Protein-engineering methods have been exploited to produce a surrogate system for the extracellular neurotransmitter-binding site of a heteromeric human ligand-gated ion channel, the glycine receptor. Acetylcholine-binding protein is a highly conserved ortholog of the pLGIC extracellular ligand-binding domain (ECD) with properties similar to nAChR. Mutations affecting key residues in the orthosteric agonist site at the α1(−)/β(+) interface affect the potency of both activation by glycine and inhibition by strychnine. We therefore set out to generate a high-fidelity surrogate of this α1(−)/β(+) orthosteric binding site using the 2α1:3β stoich­iometry [Fig. 1(a)] by exploiting protein-engineering methods and the thermal stability of acetylcholine-binding protein from Aplysia californica (AcAChBP). Ultimately, the highly stable AcAChBP framework has allowed us to introduce nine amino-acid substitutions that have resulted in a stable surrogate for a heteromeric neurotransmitter site that binds glycine.

Variants I and II presented structural features consistent with site-directed mutagenesis and electrophysiological data that suggest interacting roles for specific residues. However, our structures also emphasized that accurately replicating the α(−)/β(+) heteromeric site required changes to the β(+) side loop C, where the major differences between α-form and β-form sequences occur. Single-site substitutions were not obvious and we judged it necessary to make a major change, with four substitutions being incorporated (S206K, C207G, C208T and P209G). However, variant III co-crystallized with glycine and the ligand occupies four of the five orthosteric binding sites in the asymmetric unit. With this proof of binding we named variant III glycine-binding protein (GBP). One edge of the Tyr205 side chain helps to form one side of the binding site, with the hydroxyl group placed to donate a hydrogen bond to the carbonyl of Tyr166 (not shown), thereby linking two segments, and to accept a hydrogen bond from the glycine ligand. Tyr212 is aligned with Tyr205, creating a π-electron-rich region to interact with the glycine amino group. Solvent-mediated interactions link the Tyr212 hydroxyl with the carboxylate of Glu162 (not shown), which in turn interacts with the glycine amino group. The glycine is tucked between and participates in van der Waals interactions with the edge of Tyr205 and the face of the Trp164 indole. The glycine carboxylate is directed towards the Arg74 guanidinyl moiety, but the distances (≥3.8 Å) are too long to represent direct hydrogen-bonding interactions and a solvent-mediated association is noted.

>MLVSVYLALLVACVGQAHSQANLMRLKSDLFNRSPMYPGPTKDDPLTVTLGFFLQDIVKVDSSTNEVDLVYYERQRWKLNSLMWDPNEYGNITDFRTSAADIWTPDITAASSTRPVQVLSPQIAVVTHDGSVMFSPAQRLSFMCDPTGVDSEEGVTCAVKFESWVYSGFEIDLKTDTDQVDLSSYYASSKYEILSATQTRQVQHYKGTGEPYIDVNLVVKFRERRAGNGFFRNLFDENLYFQGHHHHHH[5x]> MTENKGIMLAKSVQKHAGRAKEKILQNLGKVDRTADEIFDDHLNNFNRQQASANRLQKEFNNYIRCVRAAQAASKTLMDSVCEIYEPQWSGYDALQAQTGASESLWADFAHKLGDQVLIPLNTYTGQFPEMKKKVEKRNRKLIDYDGQRHSFQNLQANAN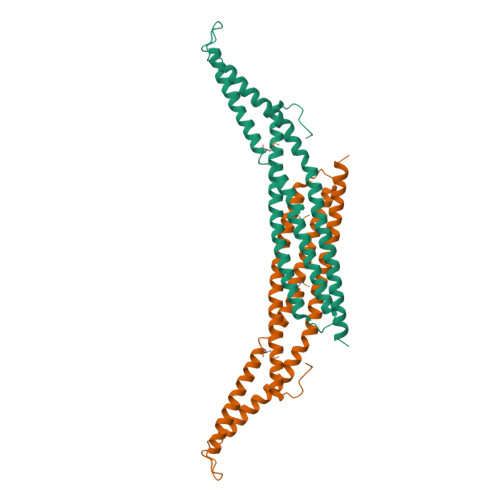KRKDDVKLTKGREQLEEARRTYEILNTELHDELPALYDSRILFLVTNLQTLFATEQVFHNETAKIYSELEAIVDKLATESQRGS Here, we investigate the function of Unc-51-like kinase 3 (ULK3), a poorly characterized member of the ULK family of serine/threonine kinases that is predicted to contain tandem MIT domains. Furthermore, our biochemical and structural studies show that the ULK3 MIT domains bind tightly to IST1, an ESCRT-III subunit required for cytokinesis. Finally, we show that ULK3 phosphorylates IST1 and other ESCRT-III proteins and that IST1 phosphorylation provides an essential inhibitory signal in the abscission checkpoint, thereby ensuring proper coordination of the final events in cell division. MIT domains bind short motifs within the C-terminal tails of ESCRT-III proteins called MIMs (MIT-interacting motifs), which become exposed and concentrated when the ESCRT-III proteins polymerize.

ULK3 residues 372–446 form the characteristic MIT three-helix bundle, and the IST1 MIM1 helix binds parallel to MIT helix 3 in the groove between MIT helices 2 and 3. The N-terminus of the MIT domain (residues 360–373) forms a short helix that packs in the groove connecting MIT helices 1 and 3. This helix has not been seen in previous MIT domain structures and is expected to interfere sterically with the binding of canonical MIM2 (and MIM3) elements. The ULK3 M434 residue is central to this interface (red), which explains why the M434D mutation inhibits IST1 binding. The additional binding energy appears to be contributed by N-terminal IST1 MIM1 residues I350 and F352, and by the central F359 residue, all of which make hydrophobic interactions that are absent in other MIM1-MIT complexes. Binding of the bulky hydrophobic IST1 MIM1 F352 and F359 residues is accommodated by complementary small ULK3 MIT2 interfacial residues A415 and G408, respectively. Charged or polar residues are found in equivalent positions of other MIT domains such as VPS4A or ULK3 MIT1. These interactions likely explain why IST1 MIM1 binds tightly and specifically to the ULK3 MIT2 domain.

> GPHMGTSARDLLREMARDKPRLLAALEVASAAMAKEEAAGGEQDALDLYQHSLGELLLLLAAEPPGRRRELLHTEVQNLMARAEYLKEQVKMRES;> TSASEDIDFDDLSRRFEELKKKT> LPTSNPAQELEARQLGRTTRDDLINGNSASCADVIFIYARGSTETGNLGTLGPSIASNLESAFGKDGVWIQGVGGAY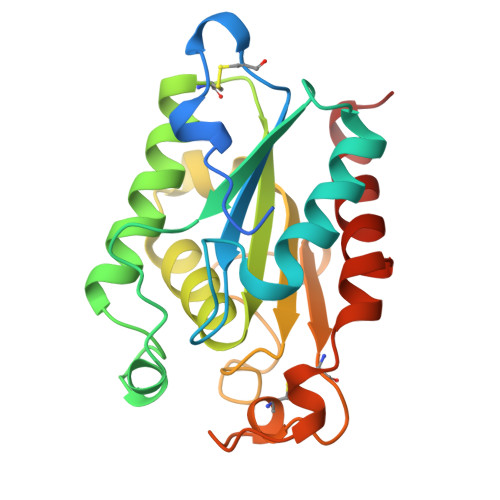RATLGDNALPRGTSSAAIREMLGLFQQANTKCPDATLIAGGYSQGAALAAASIEDLDSAIRDKIAGTVLFGYTKNLQNRGRIPNYPADRTKVFCNTGDLVCTGSLIVAAPHFAYGPDARGPAPEFLIEKVRAVRGSA>[2x]HMYANPVWTALFDYEPSGQDELALRKGDRVEVLSRDAAISGDEGWWAGQVGGQVGIFPSNYVSRGGGAIRINPNGTWSRQAETVES

MLK3, also known as MAP3K11, is a serine/threonine protein kinase involved in regulating the JNK, p38, and ERK pathways. It is composed of several modules: an SH3 domain, a kinase domain, tandem leucine zippers, a Cdc42/Rac interactive binding (CRIB) motif, several linker regions, and a proline-rich C-terminal tail. The SH3 domain has been implicated in the autoinhibition of the kinase domain through an intramolecular interaction via a nonconsensus single proline motif located between the leucine zipper and CRIB motif in the full-length MLK3 protein. The overall structure reveals a five-stranded antiparallel β-barrel, a characteristic of all known SH3 domains, and three loops (RT, n-Src, and 310 helix), commonly involved in the recognition of both proline-rich and nonproline ligands.

The newly identified binding surface is composed of an extended n-Src loop (located between β2 and β3 strands) of the MLK3 SH3 domain, which opens up to bind a peptide ligand, named “MLK3 SH3–interacting peptide” (MIP), which lacks the canonical PXXP motif. To determine the structure of the MLK3 SH3–MIP complex, we constructed a fusion protein MLK3 SH3(41–105)-MIP(1′–19′) where the prime denotes residues of the peptide. The structure of MLK3 SH3(41–105)-MIP(1′–19′) was solved to 1.2-Å resolution and refined to an Rwork/Rfree of 13.6%/15.8%. The interaction of the SH3 domain of MLK3 with MIP occurs between two protomers that are related by crystallographic symmetry. The MIP binds in a pocket formed between the n-Src loop and β-strands 2–4. Most notably, several hydrogen bonds contact Trp-10′ in the MIP sequence. The backbone amide group of Trp-10′ interacts with Asp-74, and the carbonyl group interacts with the backbone amide of Ala-76. The Trp-10′ indole nitrogen atom hydrogen bonds with the carbonyl group of Trp-83 located on the edge of β3 strand. Gly-8′ and Arg-12′ also contribute to hydrogen bonding; the carbonyl group of Gly-8′ interacts with the hydroxyl group of Ser-72 in the SH3 domain, and the guanidine moiety of Arg-12′ forms a salt bridge with the side-chain carboxylate of Asp-80. To accommodate MIP the n-Src loop undergoes a dramatic conformational change.N-{(2R)-2-[2-(hydroxyamino)-2-oxoethyl]-4-methylpentanoyl}-3-naphthalen-2-yl-L-alanyl-L-alaninamide 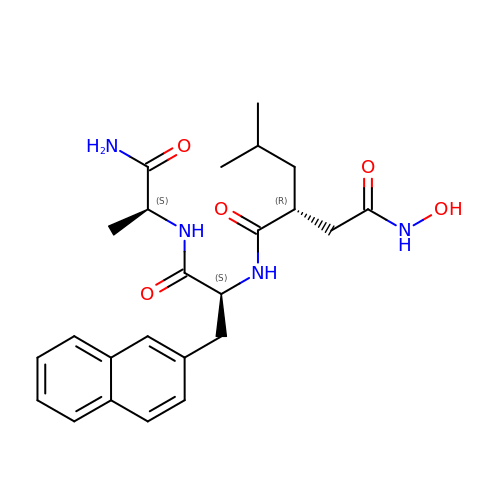| C24 H32 N4 O5 | CRCPLBFLOSEABN-BEVDRBHNSA-N>G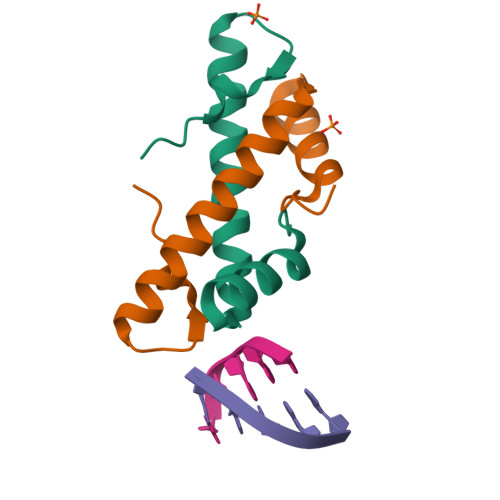HMAEVLVVTSKVKKLIKEKGQMNTSAETIDVLSKAIEQLCLKGVESAKADGRKTVMARDIVIDHL[2x]> GVITGVGGYFLFNQNKQRSSVSNFAYQPKQLSVKHQQAVDETLTPWTWNNNNFSSLKITGENPGSFGLVRSQNDNLNISSVTKNSSDDNLKYLNAVEKYLDGQQNFAIRRYDNNGRALYDINLAKMENPSTVQRGLNGEPIFDPFKGFGLTGNAPTDWNEIKGKVPVEVVQSPHSPNLYFVLLVPKVALEYHNLNNQVVKESLEVKATQSSFNPTQRLQKDSPVKDSSKQGEKLSETTASSMSSGMATSTRAKALKVEVERGSQSDSLLKNDFAKKPLKHKNSSGEVKLEAEKEFTEAWKPLLTTDQIAREKGMGATVVSFYDAPYSENHTAFGLVDHIDPKKMVENYPPSWKTPKWNHHGIWDYNARNLLLQTTGFFNPRRHPEWFDEGQAKADNTSPGFKVGDTDHKKDGFKKNSSSPIALPFEAYFANIGNMVAIGNSVFIFGGNGHATKMFTTNPLSIGVFRIKYTDNFSKSSVTGWPYAVLFGGLINPQTNGLKDLPLGTNRWFEYVPRMAVSGVKWVGNQLVLAGTLTMGDTATVPRLKYDQLEKHLNLVAQGQGLLREDLQIFTPYGWANRPDIPVGAWLQDEMGSKFGPHYFLNNPDIQDNVNNDTVEALISSYKNTDKLKHVYPYRYSGLYAWQLFNWSNKLTNTPLSANFVNENSYAPNSLFAAILNEDLLTGLSDKIFYGKENEFAENEADRFNQLLSLNPNPNTNWARYLNVVQRFTTGPNLDSSTFDQFLDFLPWIGNGKPFSNSPSPSTSASSSTPLPTFSNINVGVKSMITQHLNKENTRWVFIPNFSPDIWTGAGYRVQSANQKNGIPFEQVKPSNNSTPFDPNSDDNKVTPSGGSSKPTTYPALPNSISPTSDWINALTFTNKNNPQRNQLLLRSLLGTIPVLINKSGDSNDQFNKDSEQKWDKTETNEGNLPGFGEVNGLYNAALLHTYGFFGTNTNSTDPKIGFKADSSSSSSSTLVGSGLNWTSQDVGNLVVINDTSFGFQLGGWFITFTDFIRPRTGYLGITLSSLQDQTIIWADQPWTSFKGSYLDSDGTPKSLWDPTALKSLPNSSTTYDTNPTLSPSFQLYQPNKVKAYQTTNTYNKLIEPVDAT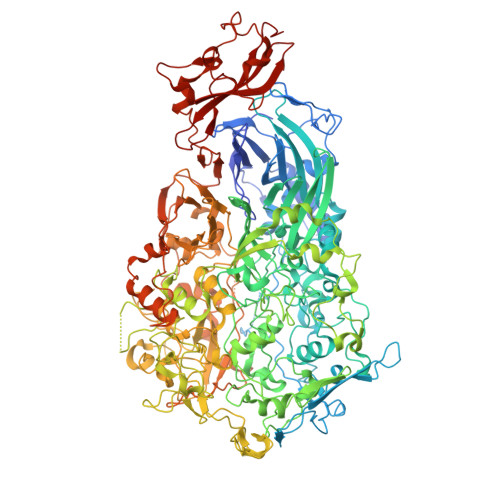SAATNMTSLLKLLTTKNIKAKLGKGTASSQGNNNGGGVSQTINTITTTGNISEGLKEETSIQAETLKKFFDSKQNNKSEIGIGDSTFTKMDGKLTGVVSTPLVNLINGQGATSDSDTEKISFKPGNQIDFNRLFTLPVTELFDPNTMFVYDQYVPLLVNLPSGFDQASIRLKVISYSVENQTLGVRLEFKDPQTQQFIPVLNASSTGPQTVFQPFNQWAHHHHHH> IVGGQECKDGECPWQALLINEENEGFCGGTILSEFYILTAAHCLYQAKRFKVRVGDRNTEQEEGGEAVHEVEVVIKHNRFTKETYDFDIAVLRLKTPITFRMNVAPACLPERDWAESTLMTQKTGIVSGFGRTHEKGRQSTRLKMLEVPYVDRNSCKLSSSFIITQNMFCAGYDTKQEDACQGDSGGPHVTRFKDTYFVTGIVSWGEGCARKGKYGIYTKVTAFLKWIDRSMK;> TRKLCSLDNGDCDQFCHEEQNSVVCSCARGYTLADNG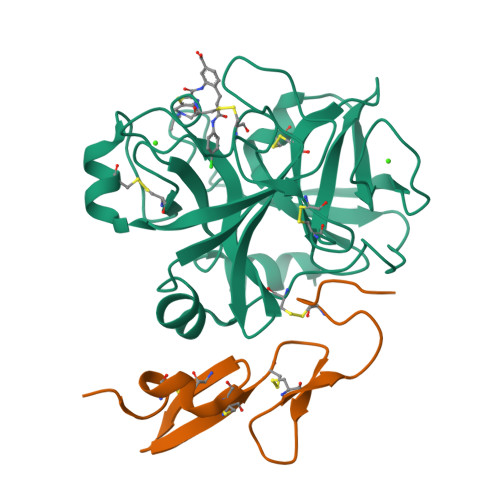KACIPTGPYPCGKQTLE Many bacterial and eukaryotic viruses with double-stranded DNA genomes in the realms Duplodnaviria and Varidnaviria encode homologs of cellular RNAPs (collectively denoted “two-barrel RNAPs”). The TMP-fused virion RNAP transcribes pre-early phage genes, including a gene that encodes another, non-virion RNAP, that transcribes early and some middle phage genes. Transcription by vRNAP and nvRNAP is directed by dissimilar AT-rich and GC-rich promoters, respectively, and the two phage RNAPs have distinct overall architectures, with the TMP-fused vRNAP being unusually flat and lacking the clamp domain.

For structural analysis of gp96 vRNAP, the shortest gp96 fragment possessing the RNAP activity was delineated using a fast cell-free assay system. The shortest fragment of gp96 that retained RNAP activity encompassed residues 327–1124. We crystallized the 1–1200 and 327–1124 fragments and determined their structures at 3.1 Å and 4.4 Å resolution, respectively. The structure of the 1–1200 fragment was largely the same as the structure of the 327–1124 fragment because most of the flanking regions not essential for the activity were disordered, except for two helices at the C-terminus (1125–1162). By contrast, the virion RNAP adopts a unique flat structure without a clamp. In contrast, gp96 vRNAP contains no defined domain at the corresponding position, resulting in a clamp-less, flat structure that heretofore has not been observed for any RNAP. We hypothesize that this unique structure enables the passage of gp96 vRNAP through the narrow channel in the phage tail. Gp96 is exceptional as it lacks the C-terminal region, and its connector element, which is disordered in the gp96 crystals (gp96 613–679), is twice shorter than in QDE-1 and phi14:2. The disordered region is likely positioned close to the RNA-DNA hybrid duplex during transcription elongation and might dynamically interact with the nascent RNA strand, moving similarly to the clamp domains of other RNAPs. We hypothesize that the vRNAP is associated with the pore formed by the TMP in the bacterial cell envelope and transcribes pre-early phage genes concomitantly with the phage genome translocation through the pore.

>[4x]MAHHHHHHSAALEVLFQGPGRNNNKPFAQQTGRFHTIELQEEGSPDEFQELLRLQASTQGHVDETTLARLVVQKRATKAILKKLLETADRPEEQAVWRAAIERLVIGNTAYDLKDDESFAKLIELAKKHPLEKVVKNVREVQFSEKVTLSDKYAFVPASNQGRIFLSHLRRENIYRTPTQRPLSLKVAEEGEGVRLKEMEEKALGDGALGILRPQSLGLPEDYTGVVQVRGELADPEGNVYAGLKGTVIVDPRAKEDFLNLNDLYRGDTVVDGKKYTKEEVDALIREKLKTGALQLNLGIHRVSTVEEAKVGKQVFLRHMGGVPFNRGRISPSEAAKWAAQAKELKFLPMIAGREMGLSHYQQIATLAKTFGVEVDEGQYSMAASHTAYKELDPEIYRLLEEGVELDAEGRPIVPIVIGKEMAAKLGLKEGDIAFTFRNPVMGHGGALLQARVAAIRDRLNAVVVNQEYAKSTGVDFDGDTLVVLPKGLPVDPHRLEVFQTLMAHAGLAGGRKGGGSVEPSPGELRFKEQLEVYDKVLARLSKSRLAAELRNAGVEDLSNPFEVVRQLESLGEEELLKAFKGYLRKGFAKELGLDLKSEEDRARLNQYLFEGFLDYRKQFQDPRRVYKKLPLMPSAALAASLLQVEAHKKEYDPSDPVALAAGQLTTSFLGLSEKLAQDLETSIDFPKLAEAIRAYNQAYSSGNEEQVAKARAELVKVLNDPTVQKFSLSNLLYQIITDRKKRDYSLRVRTESGKTYEYRNLYAVLNRLMQNLPVEEVADTVYDASGQAVEERVPLKQSATRSLVKGLLDLASGKVKEDPD>GPGSMTTPNFELYGYFRSSCSGRLRIAFHLKSIPYTRHPVNLLKGEQHSDTYKSLNPTNTVPLLVVSNINNTVSPSSASFSIGQSLAALEYLEEALPTNARPLLPPISNPVARAHVRTICNIIACDVQPVTNLKIQKKVKALDGDPTVWSRDLATQGFGAVEKLLELSAGRFC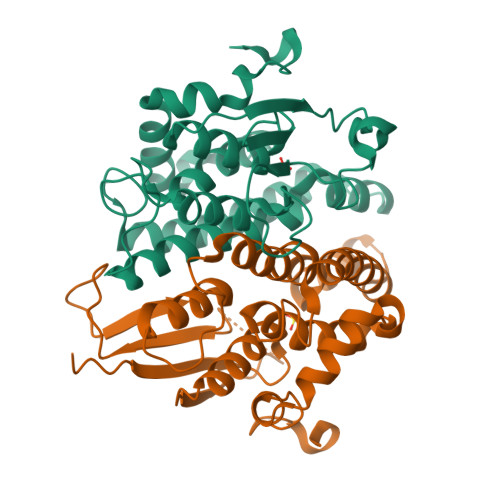VGDEITLADVCLVPAVWAAERVGMDLARFPITKRVFEEMLKEEAVQKAHWQKQEDTPEDLRA[4x]> MDPMASEIHMTGPMCLIENTNGRLMANPEALKILSAITQPMVVV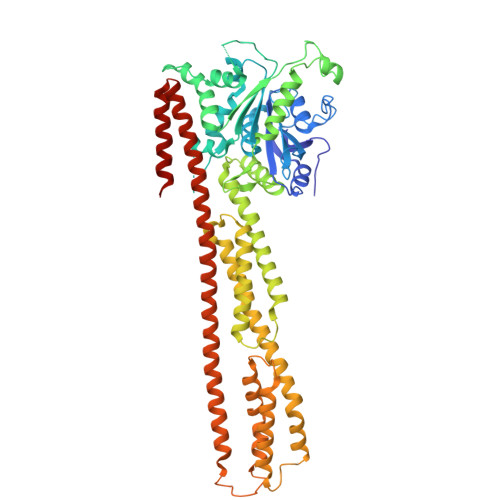AIVGLYRTGKSYLMNKLAGKKKGFSLGSTVQSHTKGIWMWCVPHPKKPGHILVLLDTEGLGDVEKGDNQNDSWIFALAVLLSSTFVYNSIGTINQQAMDQLYYVTELTHRIRSKSSPDENENEVEDSADFVSFFPDFVWTLRDFSLDLEADGQPLTPDEYLTYSLKLKKGTSQKDETFNLPRLCIRKFFPKKKCFVFDRPVHRRKLAQLEKLQDEELDPEFVQQVADFCSYIFSNSKTKTLSGGIQVNGPRLESLVLTYVNAISSGDLPCMENAVLALAQIENSAAVQKAIAHYEQQMGQKVQLPTETLQELLDLHRDSEREAIEVFIRSSFKDVDHLFQKELAAQLEKKRDDFCKQNQEASSDRCSALLQVIFSPLEEEVKAGIYSKPGGYRLFVQKLQDLKKKYYEEPRKGIQAEEILQTYLKSKESMTDAILQTDQTLTEKEKEIEVERVKAESAQASAKMLHEMQRKNEQMMEQKERSYQEHLKQLTEKMENDRVQLLKEQERTLALKLQEQEQLLKEGFQKESRIMKNEIQDLQTKMRRRKACTIS>[9x]DITVYNGQHKEAAQAVADAFTRATGIKVKLNSAKGDQLAGQIKEEGSRSPADVFYSEQIPALATLSAANLLEPLPASTINETRGKGVPV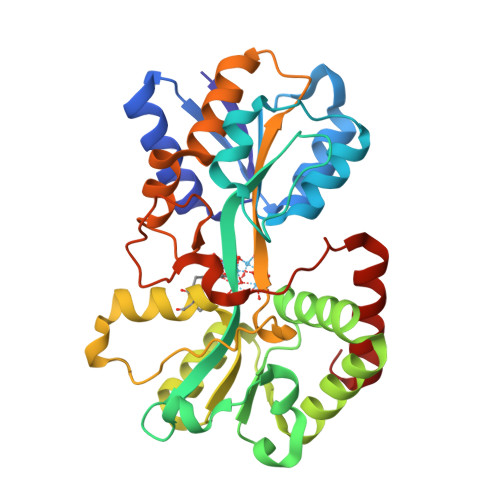AAKKDWVALSGRSRVVVYDTRKLSEKDLEKSVLNYATPKWKNRIGYVPTSGAFLEQIVAIVKLKGEAAALKWLKGLKEYGKPYAKNSVALQAVENGEVDAALINNYYWHAFAREKGVQNVHTRLNFVRHRDPGALVTYSGAAVLKSSQNKDEAKKFVAFLAGKEGQRALTAVRAEYPLNPHVVSTFNLEPIAKLEAPQVSATTVSEKEHATRLLEQAGMK> AKALIVYGSTTGNTEYTAETIARELADAGYEVDSRDAASVEAGGLFEGFDLVLLGCSTW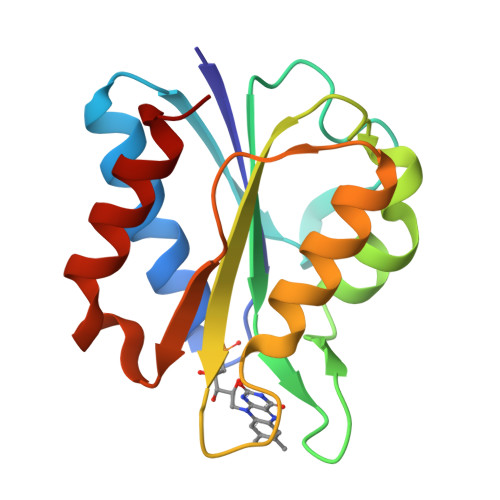GDDCIELQDDFIPLFDSLEETGAQGRKVACFGCGDSSYEYFCGAVDAIEEKLKNLGAEIVQDGLRIDGDPRAARDDIVGWAHDVRGAI>[4x]MKILKTLTLRGPNYWSIRRKKLIVMRLDLEDLAERPSNSIPGFYEGLIKVLPSLVEHFCSPGYQGGFLERVKEGTYMGHIVEHVALELQELVGMTAGFGRTRETSTPGVYNVVYEYVDEQAGRYAGRAAVRLCRSLVDTGDYPRLELEKDLEDLRDLGANSALGPSTETIVTEAEARKIPWMLLSARAMVQLGYG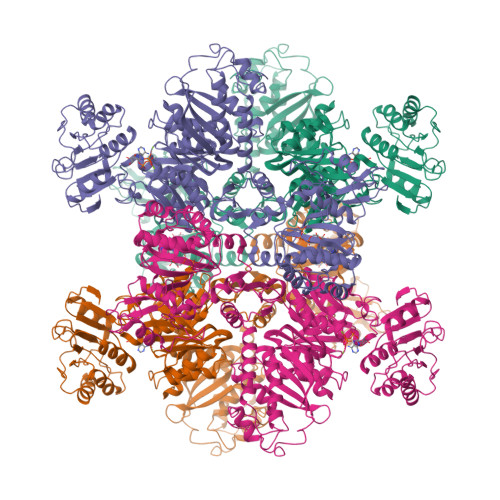VYQQRIQATLSSHSGILGVELACDKEGTKTILQDAGIPVPRGTTIQYFDDLEEAINDVGGYPVVIKPLDGNHGRGITINVRHWQEAIAAYDLAAEESKSRAIIVERYYEGSDHRVLVVNGKLVAVAERIPAHVTGDGSSTISELIEKTNQDPNRGDGHDNILTKIVVNKTAIDVMERQGYNLDSVLPKDEVVYLRATANLSTGGIAIDRTDDIHPENIWLMERVAKVIGLDIAGIDVVTSDISKPLRETNGVIVEVNAAPGFRMHVAPSQGLPRNVAAPVLDMLFPPGTPSRIPILAVTGTNGKTTTTRLLAHIYRQTGKTVGYTSTDAIYINEYCVEKGDNTGPQSAGVILRDPTVEVAVLETARGGILRAGLAFDSCDVGVVLNVAADHLGLGDIDTIEQMAKVKSVIAEVVDPSGYAVLNADDPLVAAMADKVKAKVAYFSMNPDNPIIQAHVRRNGIAAVYESGYLSILEGSWTLRVEQAKLIPMTMGGMAPFMIANALAACLAAFVNGLDVEVIRQGVRTFTTSAEQTPGRMNLFNLGQHHALVDYAHNPAGYRAVGDFVKNWQGQRFGVVGGPGDRRDSDLIELGQIAAQVFDRIIVKEDDDKRGRSEGETADLIVKGILQENPGASYEVILDETIALNKALDQVEEKGLVVVFPESVTRAIDLIKVRNPIGENLYFQ2-PHOSPHOGLYCOLIC 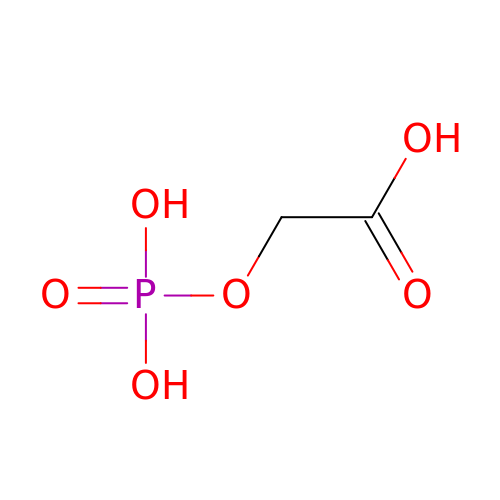ACID | C2 H5 O6 P | ASCFNMCAHFUBCO-UHFFFAOYSA-N>MGEVVRLTNSSTGGPVFVYVKDGKIIRMTPMDFDDAVDAPSWKIEARGKTFTPPRKTSIAPYTAGFKSMIYSDLRIPYPMKRKSFDPNGERNPQLRGAGLSKQDPWSDYERISWDEATDIVVAEINRIKHAYGPSAILSTPSSHHMWGNVGYRHSTYFRFMNMMGFTYADHNPDSWEGWHWGGMHMWGFSWRLGNPEQYDLLEDGLKHAEMIVFWSSDPETNSGIYAGFESNIRRQWLKDLGVDFVFIDPHMNHTARLVADKWFSPKIGTDHALSFAIAYTWLKEDSYDKEYVAANAHGFEEWADYVLGKTDGTPKTCEWAEEESGVPACEIRALARQWAKKNTYLAAGGLGGWGGACRASHGIEWARGMIALATMQGMGKPGSNMWSTTQGVPLDYEFYFPGYAEGGISGDCENSAAGFKFAWRMFDGKTTFPSPSNLNTSAGQHIPRLKIPECIMGGKFQWSGKGFAGGDISHQLHQYEYPAPGYSKIKMFWKYGGPHLGTMTATNRYAKMYTHDSLEFVVSQSIWFEGEVPFADIILPACTNFERWDISEFANCSGYIPDNYQLCNHRVIS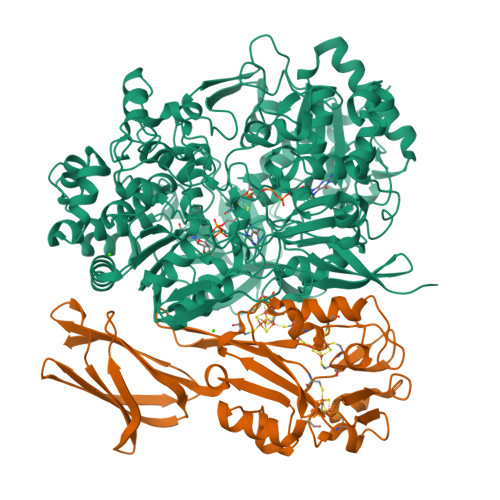LQAKCIEPVGESMSDYEIYRLFAKKLNIEEMFSEGKDELAWCEQYFNATDMPKYMTWDEFFKKGYFVVPDNPNRKKTVALRWFAEGREKDTPDWGPRLNNQVCRKGLQTTTGKVEFIATSLKNFEEQGYIDEHRPSMHTYVPAWESQKHSPLAVKYPLGMLSPHPRFSMHTMGDGKNSYMNYIKDHRVEVDGYKYWIMRVNSIDAEARGIKNGDLIRAYNDRGSVILAAQVTECLQPGTVHSYESCAVYDPLGTAGKSADRGGCINILTPDRYISKYACGMANNTALVEIEKWDGDKYEIY[12x];>[12x]MEQYYMVIDVAKCQDCNNCFMGCMDEHELNEWPGYTASMQRGHRWMNIERRERGTYPRNDINYRPTPCMHCENAPCVAKGNGAVYQREDGIVLIDPEKAKGKKELLDTCPYGVMYWNEEENVAQKCTMCAHLLDDESWAPKMPRCAHNCGSFVYEFLKTTPEAMAKKVEEEGLEVIKPELGTKPRVYYKNLYRFEKNYVTAGILVQGDCFEGAKVVLKSGGKEVASAETNFFGEFKFDALDNGEYTVEIDADGKSYSDTVVIDDKSVDLGFIKL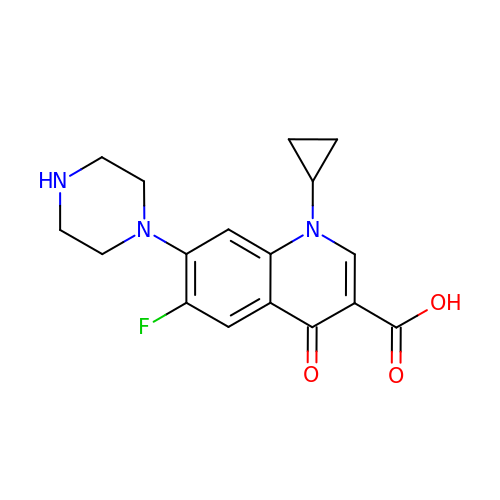1-CYCLOPROPYL-6-FLUORO-4-OXO-7-PIPERAZIN-1-YL-1,4-DIHYDROQUINOLINE-3-CARBOXYLIC ACID | C17 H18 F N3 O3 | MYSWGUAQZAJSOK-UHFFFAOYSA-N>[2x]GAMESLPVIAAPSMWTRPQIKDFKEKIQQDADSVITVGRGEVVTVRVPTHEEGSYLFWEFATDNYDIGFGVYFEWTDSPNTAVSVHVSESSDDDEEEEENIGCEEKAKKNANKPLLDE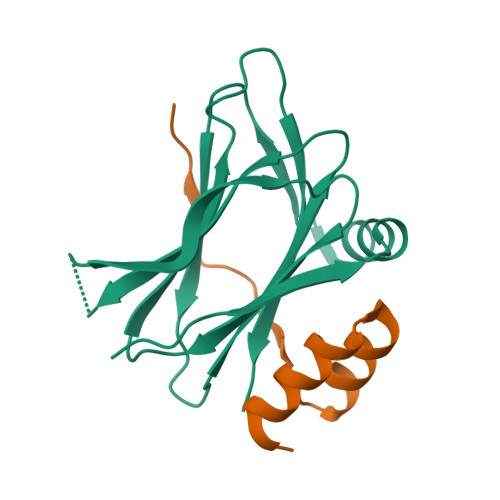IVPVYRRDCHEEVYAGSHQYPGRGVYLLKFDNSYSLWRSKSVYYRVYYTR;>[2x]GSGSGKPAPDAIGDLLASVDSEEVRQYCREQGWIIPETPTNVERHLNR> GAMGNSNSPKQIAVDPEAKELIQKILDRSEDIVQISEIDSNKGEPNDQFGMKAEIFSKIFFNANSMVHFDDNEYLNERRILYTSLNFNEGVILNLGTILSKLSQHSNYRSLVKETLINRGFSIQLAMEEISLKILNVKDKLHHLNKPNLKT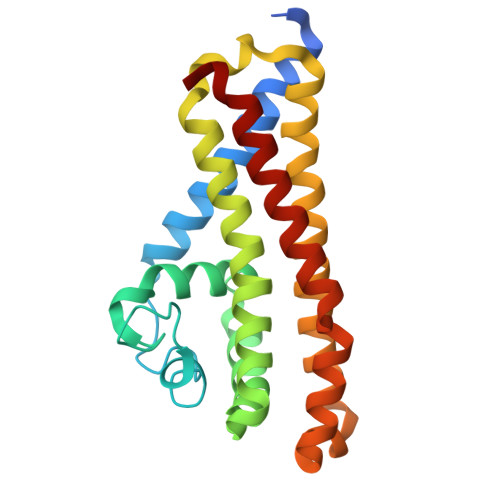LYYDFDKLKTLKEKWLKDVDDIIKEYNANPELRTNISKLHDNVELKNSKAQFADIHNLILNLINTTTNILAPIQ>GDLKTAVFNAARDGKLRLLTKLLASKSKEEVSSLISEKTNGATPLLMAARYGHLDMVEFLLEQCSASIEVGGSVNFDGETIEGAPPLWAASAAGHLKVVQSLLNHGASVNNTTLTNSTPLRAACFDGHLEIVKYLVEHKADLEVSNRHGHTCLMISCYKGHKEIAQYLLEKGADVNRKSVKGNTALHDCAESGSLDIMKMLLMYCAKMEKDGYGMTPLLSASVTGHTNIVDFLTHHAQTSKTERINALELLGATFVDKKRDLLGALKYWKKAMNMRYSDRTNIISKPVPQTLIMAYDYAKEVNSAEELEGLIADPDEMRMQALLIRERILGPSHPDTSYYIRYRGAVYADSGNFKRCINLWK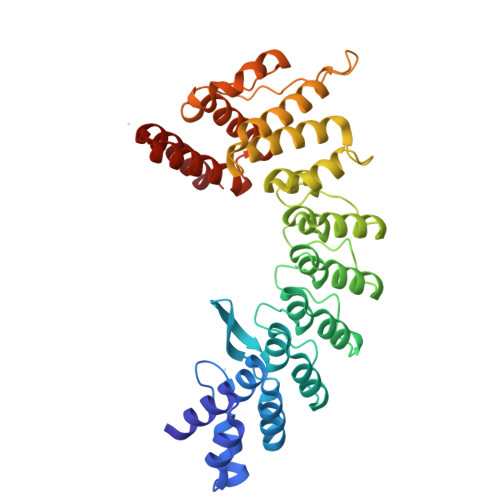YALDMQQSN[3x];>NRRRRWRERQR[3x]> METTEVIEGKNITVERTGEENRRLIFQDCLCAVCGLCGEICPVSAIEVNPTGAMVRTEQEKSKIAIDENKCVLCGMCSSICPFQALDLQIDGTSIKELAEYPKIIKSAEIDDETCIQCKACETACPQDAITITRELPERKDLVTGEIEIDKDTCIYCGMCEEMCPVDAIEIDHQTPSSASPVVATDIRVDEDKC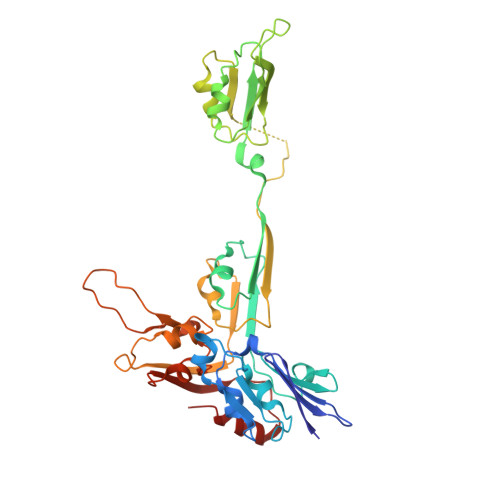VHCGICKRICPVDAIMQVCRICPYGEYEIKTPEVTGTSYIDPELCVNCGWCQEICPVDAATVTKPFEGELIIDQDTCQACETCVMVCPCNVLSFPKPEKPGEKTTKLHKDERFCIYCGACERSCPVTAITVKRNRINTTPIRSKAWKNAFDSLLK UGT76G1 is a UDP-glucose (UDPG)-dependent glycosyltransferase, where UDPG is the sugar donor and UDP is released after sugar transfer. UGT76G1 alone performs β (1–3) glycosylation of Reb D and Reb M in S. rebaudiana. Our data establish that UGT76G1 can transfer glucose in a β (1–3) manner to an existing glucose A at both the R1 and R2 positions (“ends”) of the steviol aglycone. The enzyme UGT76G1 shows an unusual degree of plasticity in substrate recognition; it is able to transfer a glucose to two different ends of some steviol glycosides despite having a single active site.

We have determined the structures of complexes of both the wild type and H25A mutant of UGT76G1 with UDP, the wild type with UDP and Reb A, and the wild type with UDP and Rubu. There is one molecule of UGT76G1 in the asymmetric unit and no stable symmetry-related multimer is identified by the PISA web server. The protein structures are all essentially identical within an r.m.s.d. of 0.4–0.9 Å over the Cα atoms. The electron density difference maps show clear density for UDP in all structures. UDP sits across the two helices Cα3 and Cα4, contacting three β-strands (Cβ3, Cβ4, and Cβ5), and is perpendicular to the central six-stranded β-sheet of the C-terminal domain. The uridine ring of UDP π-stacks against Trp 338 and forms two hydrogen bonds to the backbone (amide and carbonyl) of Val 339. The O2 and O3 hydroxyl groups of the ribose ring form a bidentate hydrogen bond with Glu 364, and a hydrogen bond forms between O3 hydroxyl and the side group amide of Asn 27. Two of the α-phosphate oxygens are bound by the main chain amides and side chains of Asn 360 and Ser 361. The pyrophosphate oxygen and two oxygen atoms of β-phosphate are linked to the NE2 of the imidazole ring of His 356 and to the amide and hydroxyl group of Ser 283, which is in the flexible loop between the Cβ1-strand and Cα1-helix. Upon Reb A or Rubu binding, the β-phosphate shows a slight shift, but the rest of UDP remains unchanged in our structures. The interactions with UDP observed here are conserved in other GT-B fold glycosyltransferases.

> MENKTETTVRRRRRIILFPVPFQGHINPILQLANVLYSKGFSITIFHTNFNKPKTSNYPHFTFRFILDNDPQDERISNLPTHGPLAGMRIPIINEHGADELRRELELLMLASEEDEEVSCLITDALWYFAQSVADSLNLRRLVLMTSSLFNFHAHVSLPQFDELGYLDPDDKTRLEEQASGFPMLKVKDIKSAYSNWQILKEILGKMIKQTKASSGVIWNSFKELEESELETVIREIPAPSFLIPLPKHLTASSSSLLDHDRTVFQWLDQQPPSSVLYVSFGSTSEVDEKDFLEIARGLVDSKQSFLWVVRPGFVKGSTWVEPLPDGFLGERGRIVKWVPQQEVLAHGAIGAFWTHSGWNSTLESVCEGVPMIFSDFGLDQPLNARYMSDVLKVGVYLENGWERGEIANAIRRVMVDEEGEYIRQNARVLKQKADVSLMKGGSSYESLESLVSYISSLLEHHHHHH>[4x]EAKKEIPLKYGATNEGKRQDPAMQKFRDNRLGAFIHWGLYAIPGGEWNGKVYGGAAEWLKSWAKVPADEWLKLMDQWNPTKFDAKKWAKMAKEMGTKYVKITTKHH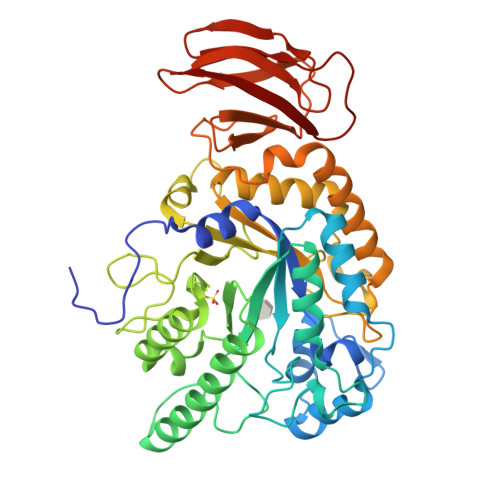EGFCLWPSKYTKYTVANTPYKRDILGELVKAYNDEGIDVHFYFSVMDWSNPDYRYDIKSKEDSIAFSRFLEFTDNQLKELATRYPTVKDFWFDGTWDASVKKNGWWTAHAEQMLKELVPGVAINSRLRADDKGKRHFDSNGRLMGDYESGYERRLPDPVKDLKVTQWDWEACMTIPENQWGYHKDWSLSYVKTPIEVIDRIVHAVSMGGNMVVNFGPQADGDFRPEEKAMATAIGKWMNRYGKAVYACDYAGFEKQDWGYYTRGKNDEVYMVVFNQPYSERLIVKTPKGITVEKATLLTTGEDITVVETTRNEYNVSVPKKNPGEPYVIQLKVRAAK>[12x]MSINSREVLAEKVKNAVNNQPVTDMHTHLFSPNFGEILLWDIDELLTYHYLVAEVMRWTDVSIEAFWAMSKREQADLIWEELFIKRSPVSEACRGVLTCLQGLGLDPATRDLQVYREYFAKKTSEEQVDTVLQLANVSDVVMTNDPFDDNERISWLEGKQPDSRFHAALRLDPLLNEYEQTKHRLRDWGY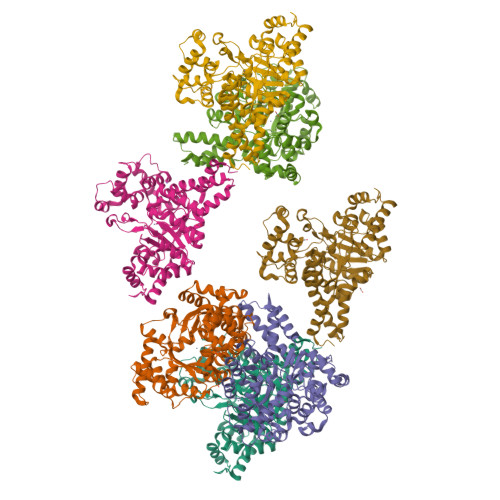KVNDEWNEGSIQEVKRFLTDWIERMDPVYMAVSLPPTFSFPEESNRGRIIRDCLLPVAEKHNIPFAMMIGVKKRVHPALGDAGDFVGKASMDGVEHLLREYPNNKFLVTMLSRENQHELVVLARKFSNLMIFGCWWFMNNPEIINEMTRMRMEMLGTSFIPQHSDARVLEQLIYKWHHSKSIIAEVLIDKYDDILQAGWEVTEEEIKRDVADLFSRNFWRFVGRNDHVTSVKVEQQT>VTSSPFKTIKSDEIFAAAQKLMPGGVSSPVRAFKSVGGQPIVFDRVKDAYAWDVDGNRYIDYVGTWGPAICGHAHPEVIEALKVAMEKGTSFGAPCALENVLAEMVNDAVPSIEMVRFVNSGTEACMAVLRIMRAYTGRDKIIKFEGCYHGHADMFLVKAGSGVATLGLPSSPGVPKKTTANTLTTPYNDLEAVKALFAENPGEIAGVILEPIVGNSGFIVPDAGFLEGLREITLEHDALLVFDEVMTGFRIAYGGVQEKFGVTPDLTTLGKIIGGGLPVGAYGGKREIMQLVA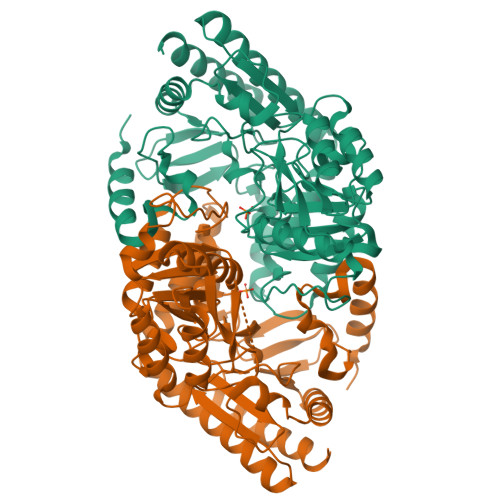PAGPMYQAGTLSGNPLAMTAGIKTLELLRQPGTYEYLDQITKRLSDGLLAIAQETGHAACGGQVSGMFGFFFTEGPVHNYEDAKKSDLQKFSRFHRGMLEQGIYLAPSQFEAGFTSLAHTEEDIDATLAAARTVMSAL[2x]>MAKIYTDKDVSLDVIKEKRVAVLGYGSQGRAWALNLRDSGIKVSVGLEREGNSWKQAENDGFKPLRTEEAVRNSDIIIFLLPDMIQRTVYLERVKPYLKEGMDLVFAHGFNIHYRLIEPPSNVDVYMIAPKAPGPIVREYFAKGGGVPALVATYQDHSGKALQKALAVAKAIGATRAGVIETTFKEETETDLFGEQVDLV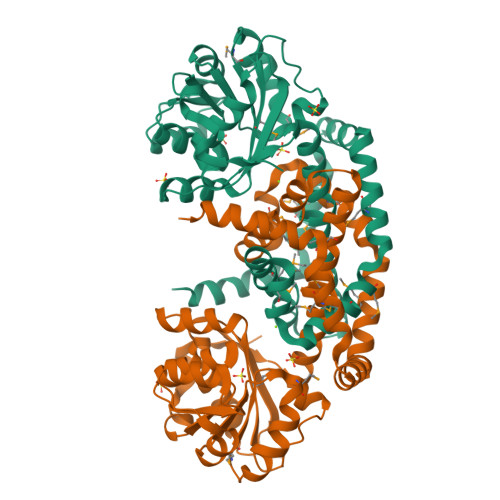GGVMQLMRYAFQTLVEAGYQPEVAYFETINEMKLIVDLVYEKGFSGMLTAVSDTAKYGGMTVGKMVIDESVKERMKKALDNIRSGKFAEKWVEEYGKGANTIKEGMKEVDNSTEEKVGRSLRDIILRGKPKSLEHHHHHH[2x]> MENAKMNSLIAQYPLVKDLVALKETTWFNPGTTSLAEGLPYVGLTEQDVQDAHARLSRFAPYLAKAFPETAATGGIIESELVAIPAMQKRLEKEYQQPISGQLLLKKDSHLPISGSIKARGGIYEVLAHAEKLALEAGLLTLDDDYSKLLSPEFKQFFSQYSIAVGSTGNLGLSIGIMSARIGFKVT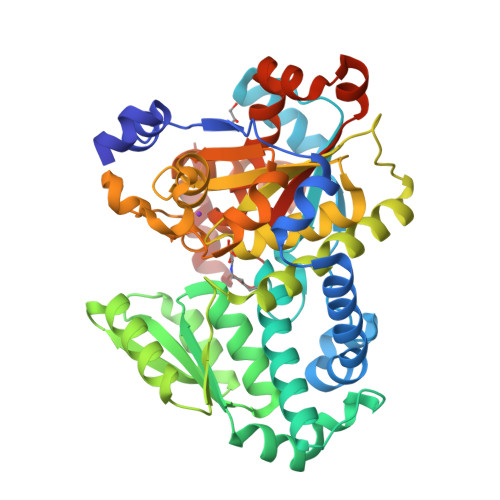VHMSADARAWKKAKLRSHGVTVVEYEQDYGVAVEEGRKAAQSDPNCFFIDDENSRTLFLGYSVAGQRLKAQFAQQGRIVDADNPLFVYLPCGVGGGPGGVAFGLKLAFGDHVHCFFAEPTHSPCMLLGVHTGLHDQISVQDIGIDNLTAADGLAVGRASGFVGRAMERLLDGFYTLSDQTMYDMLGWLAQEEGIRLEPSALAGMAGPQRVCASVSYQQMHGFSAEQLRNTTHLVWATGGGMVPEEEMNQYLAKGR>[2x]GHMSTPGAQQVLFRTGIAAVNSTNHLRVYFQDVYGSIRESLYEGSWANGTEKNVIGNAKLGSPVAATSKELKHIRVYTLTEGNTLQEFAYDSGTGWYNGGLGGAKFQVAPYSCIAAVFLAGTDALQLRIYAQKPDNTIQEYMWNGDGW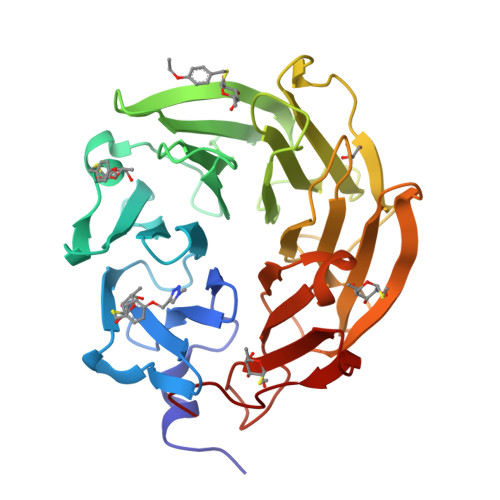KEGTNLGGALPGTGIGATSFRYTDYNGPSIRIWFQTDDLKLVQRAYDPHKGWYPDLVTIFDRAPPRTAIAATSFGAGNSSIYMRIYFVNSDNTIWQVCWDHGKGYHDKGTITPVIQGSEVAIISWGSFANNGPDLRLYFQNGTYISAVSEWVWNRAHGSQLGRSALPPA>MDFSRNLYDIGEQLDSEDLASLKFLSLDYIPQRKQEPIKDALMLFQRLQEKRMLEESNLSFLKELLFRINRLDLLITYLNTRKEEMERELQTPGRAQISAYRVMLYQISEEVSRSELRSFKGGLQEEISKCKLDDDMNLLDIFIEMEKRVILGEGKLDILKRVCAQINKSLLKIINDYEEFSKERSSSLEGSPDEFSNGEELCGVMTISDSPREQDSESQTLDKVYQMKSKPRGYCLIINNHNFAKAREKVPKLHSIRDRNGTHLDAGALTTTFEELHFEIKPHDDCTVEQIYEILKIYQLMDHSNMDCFICCILSHGDKGIIYGTDGQEAPIYELTSQFTGLKCPSLAGKPKVFFIQAAQGDNYQKGIPVETASEEQPYLEMALSSPQTRYIPDEADFLLGMATVNNCVSYRNPAEGTWYIQSLCQSLRERCPRGDDILTILTEVNYEVSNKDDKKNMGKQMPQPTFTLRKKLVFPSD[3x];>MSAEVIHQVEEALDTDEKEMLLFLCRDVAIDVVPPNVRDLLDILRERGKLSVGDLAELLYRVRRFDLLKRILKMDRKAVETHLLRNPHLVSDYRVLMAEIGEDLDKSDVSSLIFLMKDYMGRGKISKEKSFLDLVVELEKLNLVAPDQLDLLEKCLKNIHRIDLKTKIQKYKQSVQ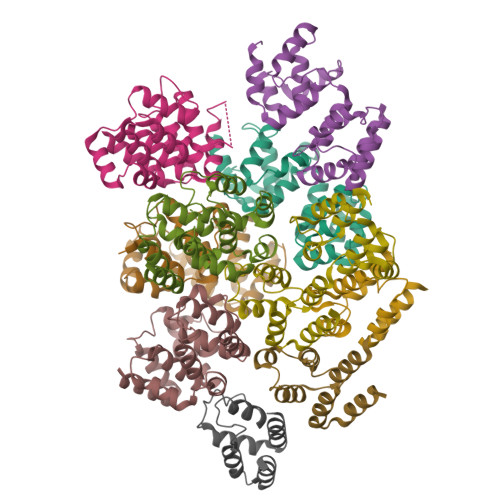GAGTS[4x];>[3x]MDPFLVLLHSVSSSLSSSELTELKFLCLGRVGKRKLERVQSGLDLFSMLLEQNDLEPGHTELLRELLASLRRHDLLRRVDDFEAGAAAGAAPGEEDLCAAFNVICDNVGKDWRRLARQLKVSDTKIDSIEDRYPRNLTERVRESLRIWKNTEKENATVAHLVGALRSCQMNLVADLVQEVQQARDLQNRSGAMSPMSWNSDASTSEASLEHHHHHH> MILITSNCARVAAFARKAACRGALCDRHRCISGGGRGD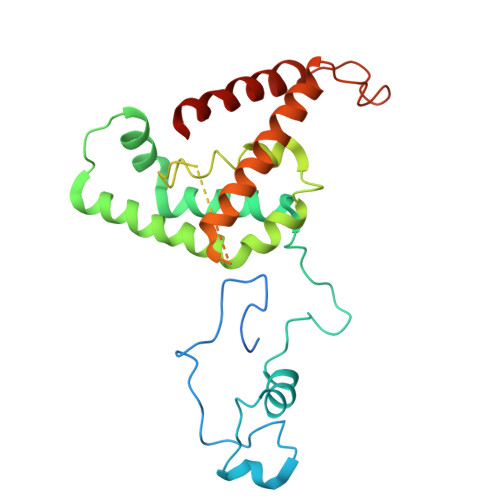LFTRHASAFKPPAFGVLRGLTHSSQTTHPQTGQLRARKLIQHAMHDRTLSGSGHHRTAVATWSYLLPSLRQNVEQAVPDTLYEKLLTDEVPLTPAESRQLADAHRLLRFELQKRIGLLEDSLADAALPYLLQWPALFQRAWLRLPMDQGSASVTDAKRDAVVPAPPSFVHAPAALPITEWAPTLSPASPSACSNGLIGRGALVPRLAQLTRHVIRCVEEDLGRLEHGSEPREDGAPRSRRQVTLEAAWRAQWASLLSWHAGTS>DNSYKMDYPEMGLCIIINNKNFHKSTGMTSRSGTDVDAANLRETFRNLKYEVRNKNDLTREEIVELMRDVSKEDHSKRSSFVCVLLSHGEEGIIFGTNGPVDLKKITNFFRGDRCRSLTGKPKLFIIQACRGTELDCGIET[2x];>CHKIPVEADFLY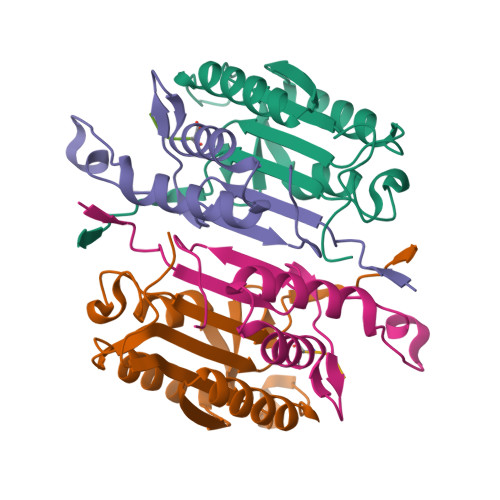AYSTAPGYYSWRNSKDGSWFIQSLCAMLKQYADKLEFMHILTRVNRKVATEFESFSFDATFHAKKQIPCIVSMLTKELYFYHH[2x];>XYKPVD[2x]>[2x]MAEQVKPAGVKPKGTVPPPKGNAPAPKANGAPGGASVIKEQDAAKMRRFLFQRTETRSTKWYQIFDTEKLDDEQVVGGHLALLGVLGFIMGIYYISGIQVFPWGAPGFHDNWFYLTIKPRMVSLGIDTYSTKTADLEAAGARLLGWAAFHFLVGSVLIFGGWRHWTHNLTNPFTGRCGNFRDFRFLGKFGDVVFNGTSAKSYKEALGPHAVYMSLLFLGWGIVMWAILGFAPIPDFQTINSETFMSFVFAVIFFALGIYWWNNPPNAAIHLNDDMKAAFSVHLTAIGYINIALGCIAFVAFQQPSFAPYYKELDKLVFYLYGEPFNRVSFNFVEQGGKVISGAKEFADFPAYAILPKSGEAFGMARVVTNLIVFNHIICGVLYVFAGVYHGGQYLLKIQLNGMYNQIKSIWITKGRDQEVQVKILGTVMALCFATMLSVYAVIVWNTICELNIFGTNITMSFYWLKPLPIFQWMFADPSINDWVMAHVITAGSLFSLIALVRIAFFAHTSPLWDDLGLKKNSYSFPCLGPVYGGTCGVSIQDQLWFAMLWGIKGLSAVCWYIDGAWIASMMYGVPAADAKAWDSIAHLHHHYTSGIFYYFWTETVTIFSSSHLSTILMIGHLVWFISFAVWFEDRGSRLEGADIQTRTIRWLGKKFLNRDVNFRFPVLTISDSKLAGTFLYFGGTFMLVFLFLANGFYQTNSPLPPPVSHAAVSGQQMLAQLVDTLMKMIA;> MAEPVENKNQAPAPGAKVPPKGAPAAPKAGAPAAPKGPVAPKAGAPAAKTGASAAKQAGKPRLASLGVTLGRSGVRQESALPYVKPKAVPPPKPAAPAAKGAPAPKGAPAAPAAKAAPGAPVAKAAPKAKKHYFIIENLCVGCGLCLDKCPPKVNAIGYKFYGDVQEGGFRCYIDQAACISCSACFSGDECPSGALIEVLPDGEVLDFSYTPPERLDFDLRFLHRFHREAR;>MDKNSNGKLIALAVGGAVLMGALFFSVSFLTGYIPAPNHSAILTPLRSFMGWFLLIFCASIIIMGLGKMSSAISDKWFLSFPLSIFVIVMVMFLSLRVYWEKGRTTTVDGKYIRTTAELKEFLNKPAATSDVPPAPAGFDFDAAKKLVDVRCNKCHTLDSVADLFRTKYKKTGQVNLIVKRMQGFPGSGISDDDAKTIGIWLHEKF[2x];> MQPQLSRPQTASNQVRKAVSGPWSGNAVHKAEKYFITSAKRDRDGKLQIELVPASGRRKLSPTPEMIRRLIDGEIEIYILTTQPDIAIDMNKEIIDMENRYVIDFDKRGVKWTMREIPVFYHEGKGLCVELHNKIYTLDQFFK;> MDAKTTILEVLKKEGKPMSAGQIAEKSGLERKEVDKAMKSLKEEELIVSPKRCYWTPKV;> MDIRRLILAFILPPAAVMNKEAGTIMLTGILTLWGWIPGVVAALIMISKEQSGKTAEA;>MALFGSNDVTTAHSDYEIVLEGGSSSWGKVKARAKVNAPPASPLLPADCDVKLNVKPLDPAKGFVRISAVFESIVDSTKNKLTIEADIANETKERRISVGEGMVSVGDFSHTFSFEGSVVNLFYYRSDAVRRNVPNPIYMQGRQFHDILMKVPLDNNDLIDTWEGTVKAIGSTGAFNDWIRDFWFIGPAFTALNEGGQRISRIEVNGLNTESGPKGPVGVSRWRFSHGGSGMVDSISRWAELFPSDKLNRPAQVEAGFRSDSQGIEVKVDGEFPGVSVDAGGGLRRILNHPLIPLVHHGMVGKFNNFNVDAQLKVVLPKGYKIRYAAPQYRSQNLEEYRWSGGAYARWVEHVCKGGVGQFEILYAQ[6x]

Upon illumination, the excitation energy is sequentially transferred from the chlorosome BChls through a monolayered baseplate, Fenna-Matthews-Olson (FMO) complexes, and ultimately to a membrane-embedded RC, where charge separation occurs. Because only one gene encodes two copies of the GsbRC core proteins (PscA subunit), the GsbRC has a homodimeric architecture with a symmetric distribution of pigments, suggesting two identical branches of electron transport chains (ETC) that could be equally utilized. Two membrane-associated PscC subunits (cytochrome cz or cyt c551) contain the cytochrome c domain, which mediates electron transfer from the menaquinol/cytochrome c oxidoreductase to the P84026–29. On the cytoplasmic surface, PscB binds two FeS clusters (FA and FB), serving as terminal electron acceptors.

However, our RC-FMO2 structure reveals the association of two FMO trimers, two PscC subunits, two accessory membrane subunits, and additional pigment molecules. In the RC-FMO2 supercomplex, the orientation of the two FMO trimers does not follow the symmetry of the PscA dimer, and each associate with the RC through a unique binding interface. The residues that contact FMO2 are more distant than those contacting FMO1, and the effective areas that contact FMO2 are much smaller than those for FMO1, resulting in a larger solvent-excluded surface for FMO1 with the membrane RC (624.0 Å2) than that for FMO2 (247.1 Å2). A BChl pigment (BChl-A816) and a monogalactosyl diglyceride (MGDG) lipid are located between PscF and PscA1. Therefore, this identified BChl is very likely to serve as a linker bacteriochlorophyll to mediate exciton transfer from FMO1 to the RC. This linker BChl is not found at the FMO2 and PscA2 interface, and the spaces between PscA2, PscC, PscE, and FMO2 are filled with lipid molecules, leaving no space for additional BChls. The linker pigment was identified along the FMO1-PscA1 axis, but not the FMO2-PscA2 axis, and this could result in a higher energy transfer efficiency in the FMO1-PscA1 pathway than the FMO2-PscA2. Also, when the RC-FMO2 structure is compared to the RC-FMO1 or the previous cryo-EM structure, a loop of PscD (Q83-P108) exhibits a slight conformational change in the presence of the second FMO trimer. Compared to the RC-FMO1 structure presented here or the previous cryo-EM structure, the RC-FMO2 structure has revealed additional pigments: one BChl a (located at the interface between FMO1 and PscA1), one F39 (located near the PscA dimer interface), and one F26 (located in the PscA2). In the RC-FMO2 supercomplex, the binding of PscB and PscD with the two FMO trimers leaves one side in the cytoplasmic space available for ferredoxin docking, and the size of this open space is sufficient for the entry of one ferredoxin molecule.> GVALHRP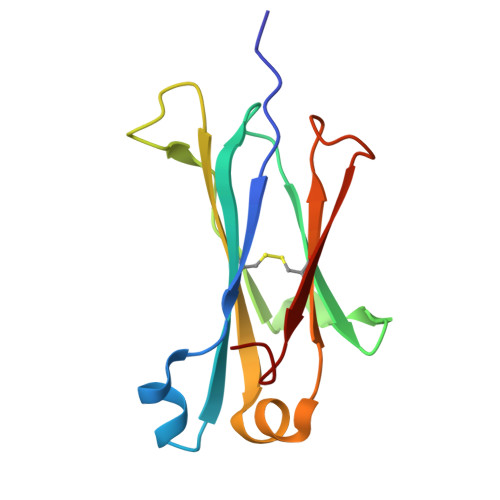DVYLLPPAREQLNLRESATITCLVTGFSPADVFVQWMQRGQPLSPEKYVTSAPMPEPQAPGRYFAHSILTVSEEEWNTGETYTCVVAHEALPNRVTERTVDKSTG CIS-4-METHYL-N-[(1S)-3-(METHYLSULFANYL)-1-(PYRIDIN-4-YLCARBAMOYL)PROPYL]CYCLOHEXANECARBOXAMIDE | 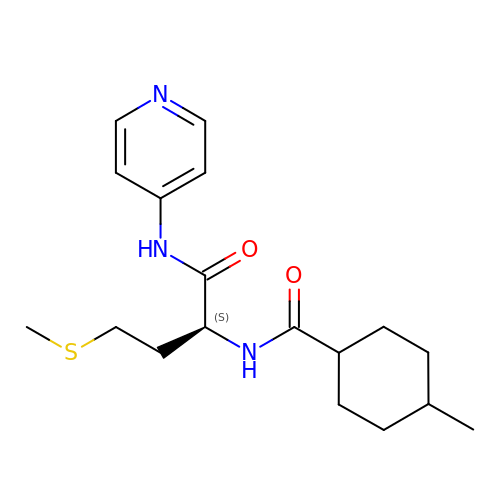C18 H27 N3 O2 S | OCZKGSPGDOPDAI-LZWOXQAQSA-N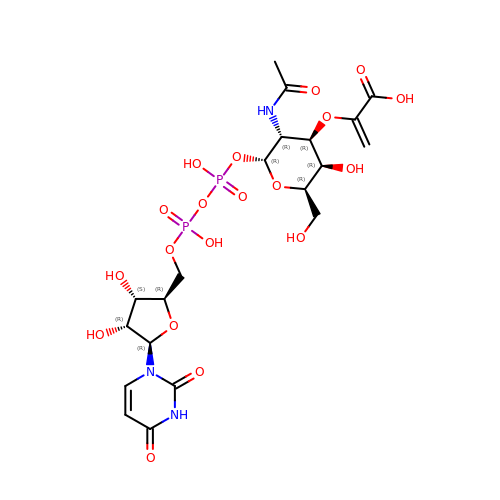2-{[(2R,3R,4R,5R,6R)-3-(acetylamino)-2-{[(S)-{[(R)-{[(2R,3S,4R,5R)-5-(2,4-dioxo-3,4-dihydropyrimidin-1(2H)-yl)-3,4-dihydroxytetrahydrofuran-2-yl]methoxy}(hydroxy)phosphoryl]oxy}(hydroxy)phosphoryl]oxy}-5-hydroxy-6-(hydroxymethyl)tetrahydro-2H-pyran-4-yl]oxy}prop-2-enoic acid | C20 H29 N3 O19 P2 | BEGZZYPUNCJHKP-ZDFMKFTCSA-N> SPSVEACGYSDRVAQLTVGNSSITTQEAANIVLAYGEWPEYCPDTDATAVDKPTRPDVSVNRFYTLDSKMWQENSTGWYWKFPDVLNKTGVFGQNAQFHYLYRSGFCLHVQCNASKFHQGALLVAVIPEFVLAGRGSNTKPNEAPHPGFNTTFPGTAGASFNDPYVLDSGVPLSQSLIYPHQWINLRTNNCATIIVPYINAVPFDSAINHSNFGLIVVPVSPLKYSSGATTAIPITVT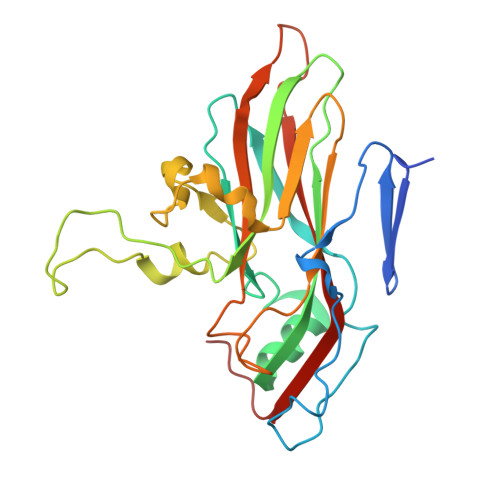IAPLNSEFGGLRQAVSQ> MTAKPTVFVVDDDMSVREGLRNLLR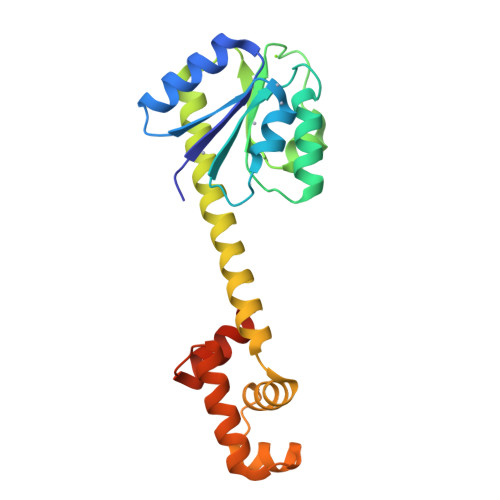SAGFEVETFDCASTFLEHRRPEQHGCLVLDMRMPGMSGIELQEQLTAISDGIPIVFITAHGDIPMTVRAMKAGAIEFLPKPFEEQALLDAIEQGLQLNAERRQARETQDQLEQLFSSLTGREQQVLQLTIRGLMNKQIAGELGIAEVTVKVHRHNIMQKLNVRSLANLVHLVEKYESFERGVS> ATGDEWWAKCKQVDVLDSEMSYYDSDPGKHKNTVIFLHGNPTSSYLWRNVIPHVEPLARCLAPDLIGMGKSGKLPNHSYRFVDHYRYLSAWFDSVNLPEKVTIVCHDWGSGLGFHWCNEHRDRVKGIVHMESVVDVIESWDEWPDIEEDIALIKSEAGEEMVLKKNFFIERLLPSSIMRKLSEEEMDAYREPFVEPGESRRPTLTWPREIPIKGDGPEDVIEIVKSYNKWLSTSKDIPKLFINADPGFFSNAIKKVTKNWPNQKTVTVKGLHFLQEDSPEEIGEAIADFLNELT

The light-producing reaction catalysed by the Renilla-type luciferase is one of the most widely used biochemical reactions in molecular and cell biology research. Here we track the role of dynamics in evolution, starting from the evolvable and thermostable ancestral protein AncHLD-RLuc which catalyses both dehalogenase and luciferase reactions. The regions encompassing the L9-α4 fragment and L14 loop are important structural elements that line the main access tunnels connecting the buried active site to the surrounding solvent. We conclude that the LUC activity benefits from conformational dynamics of the protein’s rigid scaffold to allow binding of a bulky substrate.

To verify the importance of the hotspot regions highlighted by biophysical analysis, we transplanted the sequence corresponding to the L9-α4 fragment from the modern RLuc8 enzyme into the ancestral AncHLD-RLuc. The resulting AncFT protein had lower thermal stability than the ancestral variant (with ca. 7 °C lower Tm value) but folded correctly (with a CD spectrum similar to that of AncHLD-RLuc and AncINS). Most importantly, both the active site cavity and the α4 helix conformation of AncFT are more open than in AncHLD-RLuc, AncINS, and even the RLuc8 chain B. Transplantation of the L9-α4 flexible region from RLuc8 into the scaffold of AncHLD-RLuc affected substrate-binding kinetics: AncFT was found to have comparable initial collision kinetics to AncINS and RLuc8, but the fragment transplantation enhanced the following conformational change and (unlike AncINS) AncFT reached the overall binding efficiency of the modern luciferase. Similar values of the specificity constant kcat/Km were obtained for AncFT and RLuc8, indicating comparable efficiency of substrate binding. Thus, AncFT’s lower LUC activity is due to a lower rate of the chemical transformation (i.e., the step after binding), as indicated by a 10-fold lower kcat value for AncFT compared to RLuc8. On the other hand, AncFT exhibited markedly weaker product inhibition than RLuc8. The half-life (t1/2) of AncFT bioluminescence was two orders of magnitude longer than that of RLuc8, being consistent with a significantly lower Km/Kp ratio determined for AncFT, in comparison to RLuc8. MD simulations of AncFT revealed that the B-factor profile of its cap domain closely resembled that of RLuc8. Based on MD simulations and HDX-MS experiments, we conclude that the transplantation reduced motions of the L9 loop, but increased motion of the α4-α5′ helices, making the mutant protein’s dynamics more similar to RLuc8.> MD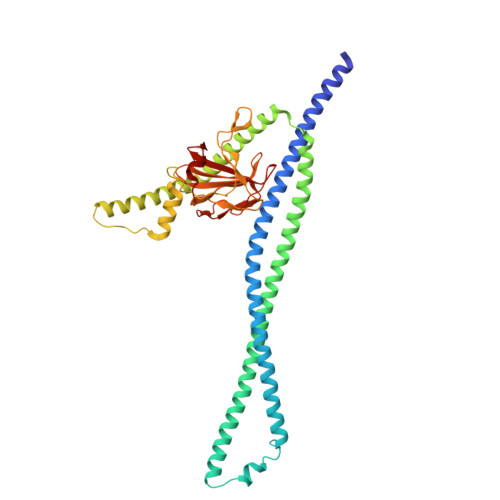ERDQLKSIQADIAAKERAVRQKQQQRASLLAQLKKQEEAISEATRKLRETQNTLNQLNKQIDEMNASIAKLEQQKAAQERSLAAQLDAAFRQGEHTGIQLILSGEESQRGQRLQAYFGYLNQARQETIAQLKQTREEVAMQRAELEEKQSEQQTLLYEQRAQQAKLTQALNERKKTLAGLESSIQQGQQQLSELRANESRLRNSIARAEAAAKARAEREAREAQAVRDRQKEATRKGTTYKPTESEKSLMSRTGGLGAPRGQAFWPVRGPTLHRYGEQLQGELRWKGMVIGASEGTEVKAIADGRVILADWLQGYGLVVVVEHGKGDMSLYGYNQSALVSVGSQVRAGQPIALVGSSGGQGRPSLYFEIRRQGQAVNPQPWLGR> M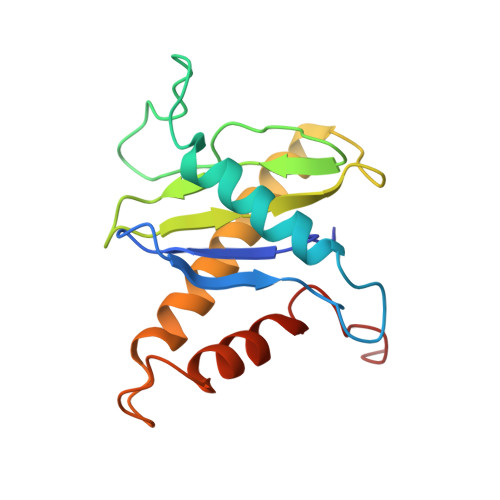SLRPCFVSLIDESDKPILIYVPNEAENEMNDVLKYNVLSNISLDYFESALVEWHSLDSKPLLKSIFQLEGVSVFAMLIKQTGLKIVIGFEQKSLSGADDEFEAINQIFETVRKIYIRVKCNPLLVSGDEKSIIKSLERKFDELFISTEVEL>[2x]MSLKRILIVDDDTAILDSTKQILEFEGYEVEIAATAGEGLAKIENEFFNLALF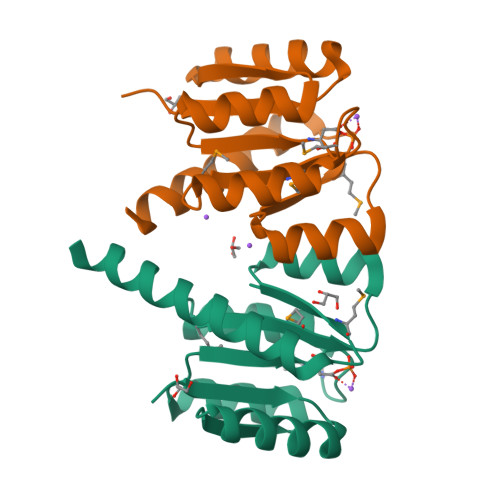DIKLPDMEGTELLEKAHKLRPGMKKIMVTGYASLENSVFSLNAGADAYIMKPVNPRDLLEKIKEKLDEQEKEGHHHHHH> MRT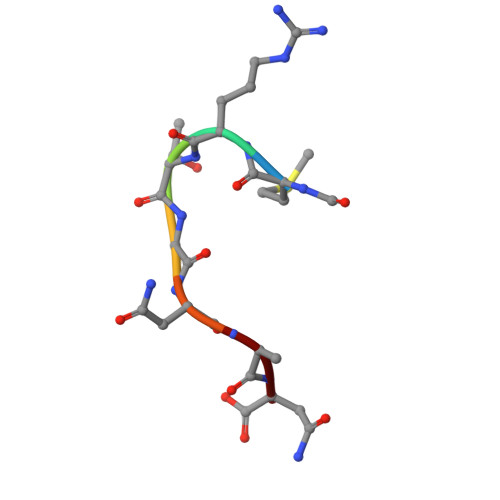GNAN>ETQSFNFDHFEENSKELNLQRQASIKSNGVLELTKLTKNGVPVWKSTGRALYAEPIKIWDSTTGNVASFETRFSFNITQPYAYPEPADGLTFFMVPPNSPQGEDGGNLGVFKPPEGDNAFAVEFDTFQNTWDPQVPHIGID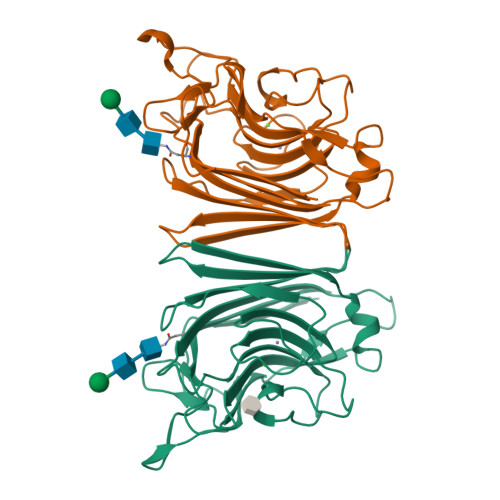VNSIVSSKTLHFQLENGGVANVVIKYDSPTKILNVVLAFHSVGTVYTLSNIVDLKQEFPNSEWVNVGLSATTGYQKNAVETHEIISWSFTSSLQETN[2x]> MAHHHHHHADLPIMHDSDRYELVKDIGSGNFGVARLMRDKQSNELVAVKYIERGEKIDENVKREIINHRSLRHPNIVRFKEVILTPTHLAIVMEYASGGEL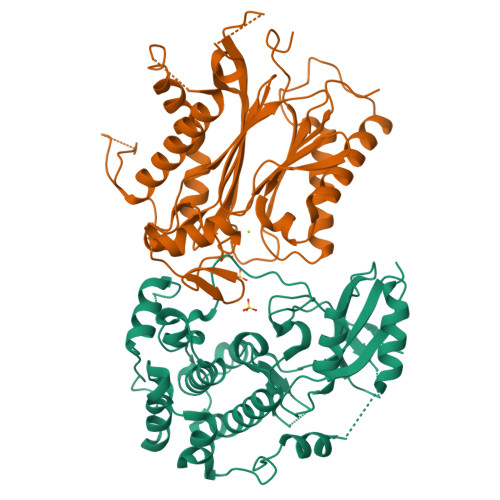FERICNAGRFSEDEARFFFQQLISGVSYCHAMQVCHRDLKLENTLLDGSPAPRLKICDFGYSKSSVLHSQPKSTVGTPAYIAPEVLLKKEYDGKVADVWSCGVTLYVMLVGAYPFEDPEEPKNFRKTIHRILNVQYAIPDYVHISPECRHLISRIFVADPAKRISIPEIRNHEWFLKNLPADLMNDNTMTTQFAASDQPGQSIEEIMQIIAEATVPPAGTQNLNHYLTGSLDIDDDMEEDLESDLDDLDIDSSGEIVYAM;> GSGSAGSAAGSNHLVKGRSVYELDCIPLWGTVSIQGNRSEMEDAFAVSPHFLKLPIKMLMGDHEGMSPSLTHLTGHFFGVYDGHGGHKVADYCRDRLHFALAEEIERIKDELCKRNTGEGRQVQWDKVFTSCFLTVDGEIEGKIGRAVVGSSDKVLEAVASETVGSTAVVALVCSSHIVVSNCGDSRAVLFRGKEAMPLSVDHKPDREDEYARIENAGGKVIQWQGARVFGVLAMSRSIGDRYLKPYVIPEPEVTFMPRSREDECLILASDGLWDVMNNQEVCEIARRRILMWHKKNGAPPLAERGKGIDPACQAAADYLSMLALQKGSKDNISIIVIDLKAQRKFKTRT7-{8-chloro-11-[3-(4-chloro-3,5-dimethylphenoxy)propyl]-1-oxo-7-(1,3,5-trimethyl-1H-pyrazol-4-yl)-4,5-dihydro-1H-[1,4]diazepino[1,2-a]indol-2(3H)-yl}-1-methyl-1H-indole-3-carboxylic acid | C39 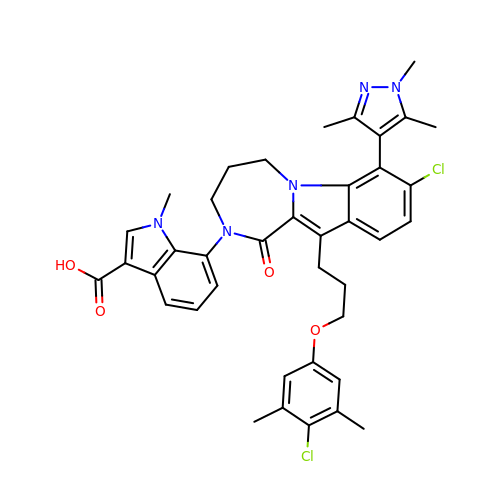H39 Cl2 N5 O4 | SIUYYHMJPRXSEZ-UHFFFAOYSA-N>[2x]SNAMTDEIDSDANNTHELTAEVARALIARGWRLTTAESCTGGNLAAALCAQADTAAFYDTGVVTFSDEAKRNVLQVRAETL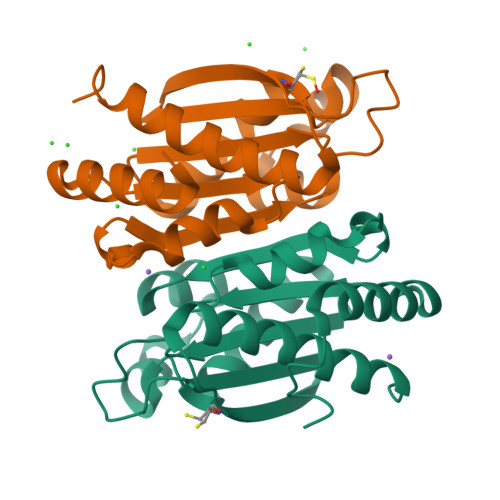AVHSAVSEACVQEMSSGILALAGADIAIAVSGYAGPEGGEDGTPAGTVWFAWNFRGQTETKRMCFAGDCETVVAKAVRYALAALSEKLAHWQ> GSMEEEAETEEQQRFSYQQRLKAAVHYTVGCLCEEVA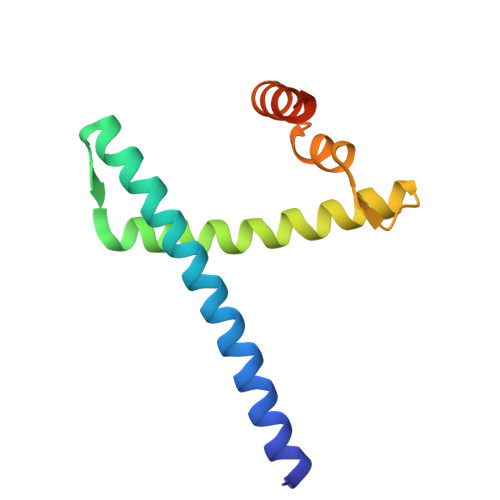LDKEMQFSKQTIAAISELTFRQCENFAKDLEMFARHAKRTTINTEDVKLLARRSNSLLKYITDKSEEIAQINLER> SANNPWTGFQIFLSPYYANEVAAAAKQITDPTLSSKAASVANIPTFTWLDSVAKIPDLGTYLASASALGKSTGTKQLVQIVIYDLPDRDCAAKAVNGEFSIANNGQANYENYIDQIVAQIQQFPDVRVVAVIEPDSLANLVTNLNVQKCANAKTTYLASVNYALTNLAKVGVYMYMDAGHAGWLGWPANLSPAAQLFTQVWQNAGKSPFIKGLATNVANYNALQAASPDPITQGNPNYDEIHYINALAPLLQQAGWDATFIVDQGRSGVQNIRQQW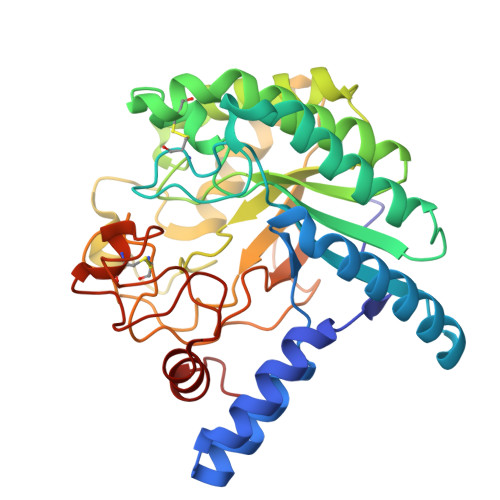GDWCNIKGAGFGTRPTTNTGSQFIDSIVWVKPGGESDGTSNSSSPRYDSTCSLPDAAQPAPEAGTWFQAYFQTLVSAANPPL>GMGFLDALMGNASEVDLGK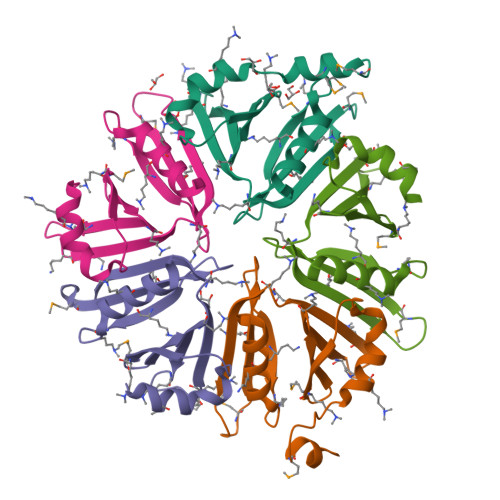LAAELSPILGDNEELQLAYKMVRDLFVFTSKRLILIDKQGVTGKKVSYHSIPYKAIVHFQVETAGTFDMDAELKLWISGQHEPLVKELKRGTDVVGIQKTIARYALG[5x]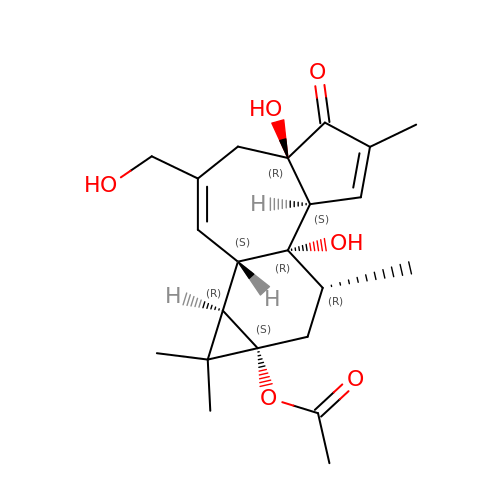prostratin | C22 H30 O6 | BOJKFRKNLSCGHY-HXGSDTCMSA-N> GGLEKDFLPLYFGWFLTKKSSETLRKAGQVFLEELGNHKAFKKELRHFISGDEPKEKLELVSYFGKRPPGVLHCTTKFCDYGKAAGAEEYAQQEVVKRSYGKAFKLSISALFVTPKTAGAQVVLTDQELQLWPSDLDKPSASEGLPPGSRAHVTLGCAADVQPVQTDLDLLDILQQVKGG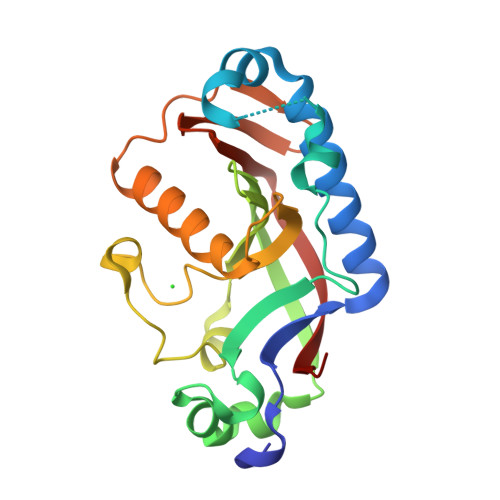SQGEAVGELPRGKLYSLGKGRWMLSLTKKMEVKAIFTGYYG pmcGlucose-6-phosphate dehydrogenase (G6PD) is a housekeeping enzyme that generates NADPH. G6PD exists as a monomer, homodimer, and homotetramer, with each monomer having three binding sites: one for catalytic glucose-6-phosphate (G6P), one for an NADP+ cofactor, and an allosteric NADP+-binding site. The latter allosteric NADP+-binding site, also known as the structural NADP+-binding site, is important for maintaining long-term protein stability and for promoting oligomer assembly. Oligomerization is central to G6PD function as it controls the activity of G6PD; the monomer is inactive with both the dimer and tetramer being the active forms.

Structurally, lysine 403 (K403), forms an important contact with a phosphate group of the structural NADP+, and studies by Wang et al. revealed that K403 is acetylated in RBCs under physiological conditions. Mutation of K403 to glutamine (K403Q) mimics acetylation, with both acetylation and K403Q disrupting oligomerization and G6PD activity in cells. Firstly, and consistent with our hypothesis, the mutation of lysine to glutamine disrupted structural NADP+ binding—no density was observed for structural NADP+. Additionally, no density was observed for the ßM and ßN strands of the structural NADP+-binding site (shown in black on G6PDWT in Fig. 3A), which caused major changes in the globular structure of the dimer (white to salmon). Secondly, major alterations were observed in the αf-helix; the αf-helix was extended, causing a loop to protrude into the G6P-binding pocket. However, in G6PDK403Q, the αj-helix is shifted, preventing K290/E287 and E347/K275 salt bridges from forming, explaining loss of tetramerization. Therefore, we solved the protein structure for G6PDK403Q and confirmed that major structural alterations occur in the G6PDK403Q dimer: the structural NADP+ is not bound, the catalytic G6P-binding site is occluded, and there are major changes in the globular structure of the dimer. These observations explain our biochemical data; G6P occlusion hinders G6PD activity, and dimer distortion prevents salt-bridge interactions at the tetramer interface, and these findings are consistent with previous structures solved for Class I variants. Interestingly, although G6PDK403Q forms a dimer that is less prone to dissociation, it is inactive and thermally unstable. It should be noted that the resolution of G6PDK403Q is relatively low, 3.65-Å, with the crystallographic structure having high B-factors.

> MAEQVALSRTQVCGILREELFQGDAFHQSDTHIFIIMGASGDLAKKKIYPTIWWLFRDGLLPENTFIVGYARSRLTVADIRKQSEPFFKATPEEKLKLEDFFARNSYVAGQYDDAASYQRLNSHMNALHLGSQANRLFYLALPPTVYEAVTKNIHESCMSQIGWNRIIVEKPFGRDLQSSDRLSNHISSLFREDQIYRIDHYLGKEMVQNLMVLRFANRIFGPIWNRDNIACVILTFKEPFGTEGRGGYFDEFGIIRDVMQNHLLQMLCLVAMEKPASTNSDDVRDEKVKVLKCISEVQANNVVLGQYVGNPDGEGEATKGYLDDPTVPRGSTTATFAAVVLYVENERWDGVPFILRCGKALNERKAEVRLQFHDVAGDIFHQQCKRNELVIRVQPNEAVYTQMMTKKPGMFFNPEESELDLTYGNRYKNVKLPDAYERLILDVFCGSQMHFVRSDELREAWRIFTPLLHQIELEKPKPIPYIYGSRGPTEADELMKRVGFQYEGTYKWVNPHKL> MADVPKREVENVEFVF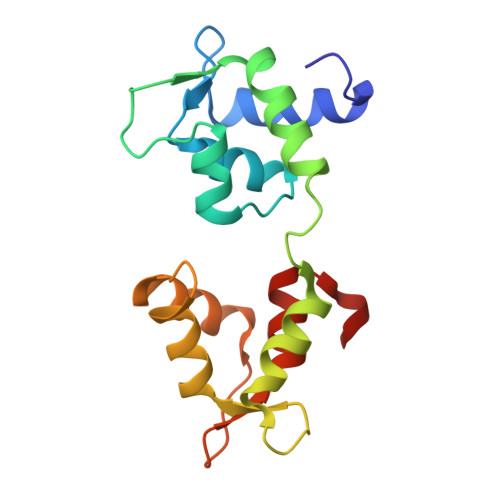EVMGSPGEGIDAVDLGDALRALNLNPTLALIEKLGGTKKRNEKKIKLDEFLPIYSQVKKEKEQGCYEDFIECLKLYDKEENGTMLLAELQHALLALGESLDDEQVETLFADCMDPEDDEGFIPYSPFLARMCDRPDQLK> MKEFYLTVEQIGDSIFERYIDSNGRERTREVEYKPSLFAHCPESQATKYFDIYGKPCTRKLFANMRDASQWIKRMEDIGLEALGMDDFKLAYLSDTYNYEIKYDHTKIRVANFDIEVTSPDGFPEPSQAKHPIDAITHYDSIDDRFYVFDLLNSPYGNVEEWSIEIAAKLQEQGGDEVPSEIIDKIIYMPFDNEKELLMEYLNFWQQKTPVILTGWNVESFAIPYVY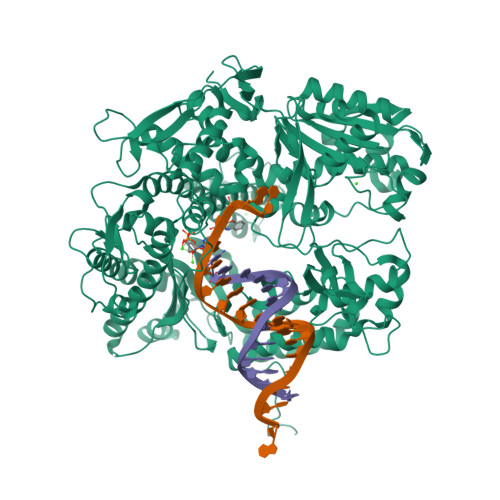NRIKNIFGESTAKRLSPHRKTRVKVIENMYGSREIITLFGISVLDYIDLYKKFSFTNQPSYSLDYISEFELNVGKLKYDGPISKLRESNHQRYISYNIIAVYRVLQIDAKRQFINLSLDMGYYAKIQIQSVFSPIKTWDAIIFNSLKEQNKVIPQGRSHPVQPYPGAFVKEPIPNRYKYVMSFDLTSLYPSIIRQVNISPETIAGTFKVAPLHDYINAVAERPSDVYSCSPNGMMYYKDRDGVVPTEITKVFNQRKEHKGYMLAAQRNGEIIKEALHNPNLSVDEPLDVDYRFDFSDEIKEKIKKLSAKSLNEMLFRAQRTEVAGMTAQINRKLLINSLAGALGNVWFRYYDLRNATAITTFGQMALQWIERKVNEYLNEVCGTEGEAFVLYGDTDSIYVSADKIIDKVGESKFRDTNHWVDFLDKFARERMEPAIDRGFREMCEYMNNKQHLMFMDREAIAGPPLGSKGIGGFWTGKKRYALNVWDMEGTRYAEPKLKIMGLETQKSSTPKAVQKALKECIRRMLQEGEESLQEYFKEFEKEFRQLNYISIASVSSANNIAKYDVGGFPGPKCPFHIRGILTYNRAIKGNIDAPQVVEGEKVYVLPLREGNPFGDKCIAWPSGTEITDLIKDDVLHWMDYTVLLEKTFIKPLEGFTSAAKLDYEKKASLFDMF> XPHEMCYWADAYCRYS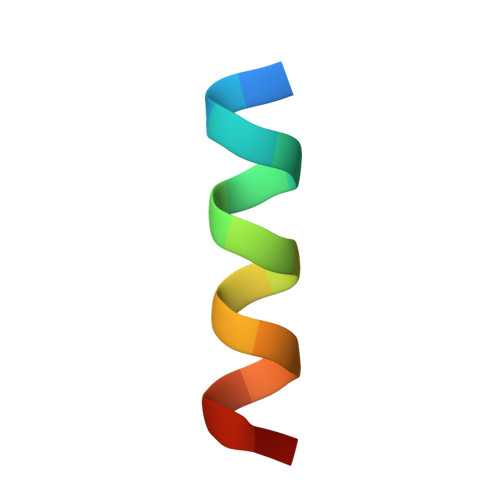X> GSHMGTRDDEYDYLFKVVLIGDSGVGKSNLLSRFTRNEFNLESKSTIGVEFATRSIQVDGKTIKAQIWDTAGLERYRAITSAYYRGAVG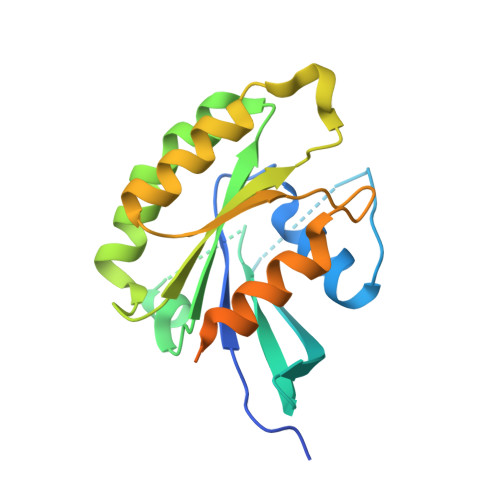ALLVYDIAKHLTYENVERWLKELRDHADSNIVIMLVGNKSDLRHLRAVPTDEARAFAEKNGLSFIETSALDSTNVEAAFQTILTEIYRIVSQKQMSDRRENDMSPSNNVVPIHVPPTTENKPKVQCCQNI> DVSFRLSGATSSSYGVFISNLRKALPNERKLYDIPLLRSSLPGSQRYALIHLTNYADETISVAIDVTNVYIMGYRAGDTSYFFNRASATEAAKYVFKDAMRK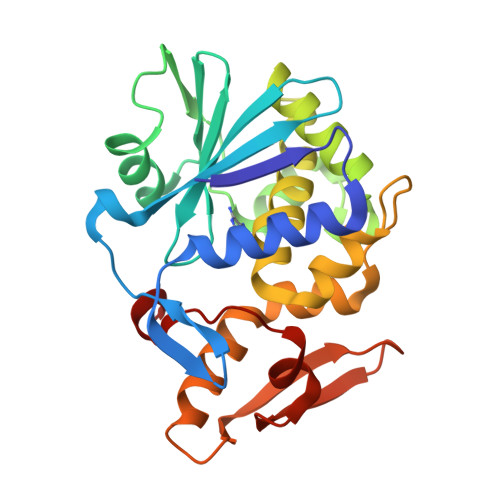VTLPYSGNYERLQTAAGKIRENIPLGLPALDSAITTLFYYNANSAASALMVLIQSTSEAARYKFIEQQIGKRVDKTFLPSLAIISLENSWSALSKQIQIASTNNGQFESPVVLINAQNQRVTITNVDAGVVTSNIALLLNRNNMA> GPKQKIVIKATMSNAKSRAQAMVLASKANGVGSVGITGDLKDQLEVVG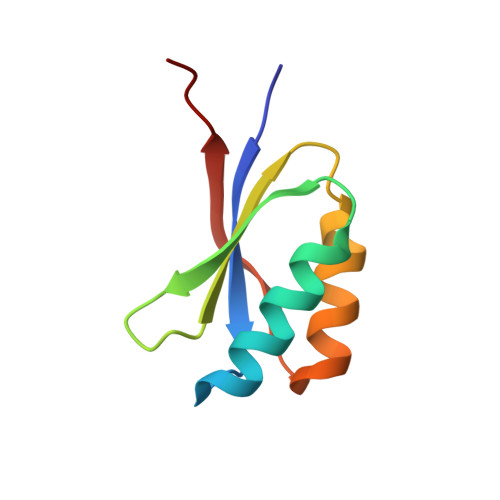VGIDIACLVRCLRKKLRYAEIVKVEEVKDK> MSHHHHHHSSQGGPQDHVEIIPLGGMGEIGKNITVFRFRDEIFVLDGGLAFPEEGMPGVDLLIPRVDYLIEHRHKIKAWVLTHGAEDHIGGLPFLLPMIFGKESPVPIYGARLTLGLLRGKLEEFGLRPGAFNLKEISPDDRIQVGRYFTLDLFRMTHSIPDNSGVVIRTPIGTIVHTGDFKLDPTPIDGKVSHLAKVAQAGAEGVLLLIADATNAERPGYTPSEMEIAKELDRVIGRAPGRVFVTTFASHIHRIQSVIWAAEKYGRKVAMEGRSMLKFSRIALELGYLKVKDRLYTLEEVKDLPDHQVLILATGSQGQPMSVLHRLAFEGHAKMAIKPGDTVILSSSPIPGNEEAVNRVINRLYALGAYVLYPPTYKVHASGHASQEELKLILN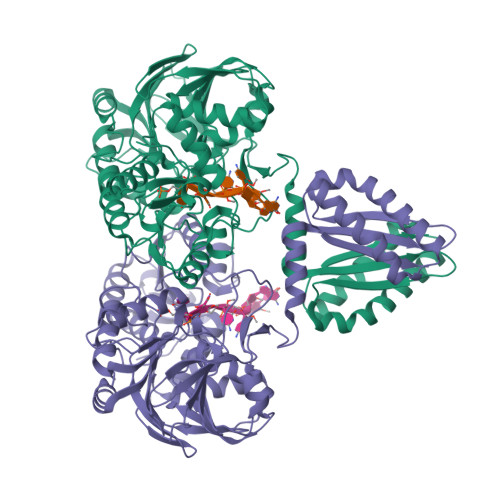LTTPRFFLPWHGEVRHQMNFKWLAESMSRPPEKTLIGENGAVYRLTRETFEKVGEVPHGVLYVDGLGVGDITEEILADRRHMAEEGLVVITALAGEDPVVEVVSRGFVKAGERLLGEVRRMALEALKNGVREKKPLERIRDDIYYPVKKFLKKATGRDPMILPVVIE>[8x]LGTNYLLSGQTLNTDGHLKNGDFDLVMQNDCNLVLYNGNWQSNTANNGRDCKLTLTDY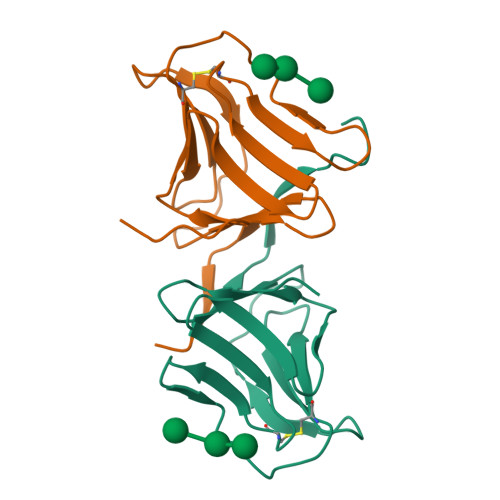GELVIKNGDGSTVWRSRAKSVKGNYAAVLHPDGRLVVFGPSVFKIDPWVPGL;>[8x]NIPFTDNLLFSGQVLYGDGRLTAKNHQLVMQGDCNLVLYGGKYGWQSNTHGNGEHCFLRLNHKGELIIKDDDFKTIWSSNSSSKQGDYVLILRDDGFAVIYGPAIWETSA>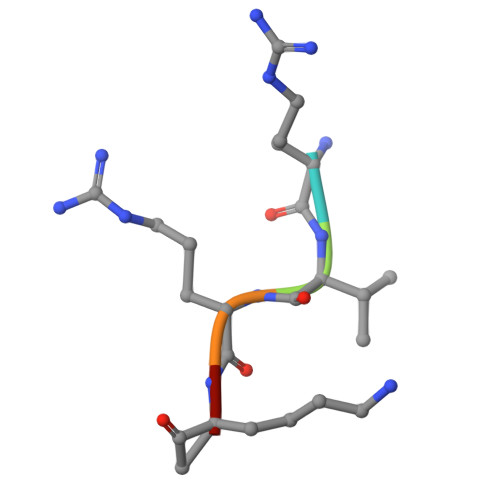 RVRKX>[3x]MPCSEETPAISPSKRARPAEVGGMQLRFARLSEHATAPTRGSARAAGYDLYSAYDYTIPPMEKAVVKTDIQIALPSGCYGRVAPRSGLAAKHFIDVGA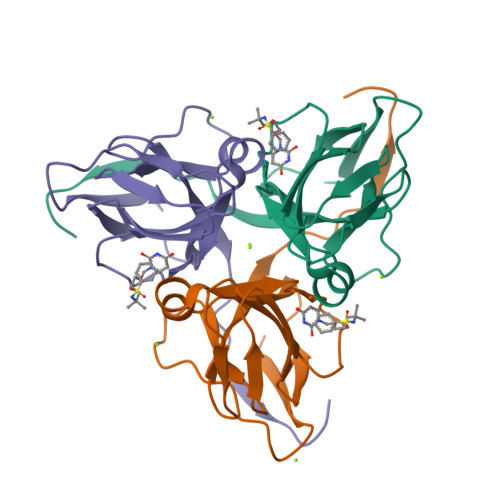GVIDEDYRGNVGVVLFNFGKEKFEVKKGDRIAQLICERIFYPEIEEVQALDDTERGSGGFGSTGKN>[2x]MVPISPIETVPVKLKPGMDGPKVKQWPLTEEKIKALVEICTEMEKEGKISKIGPENPYNTPVFACKKKDSTKWRKLVDFRELNKRTQDFWEVQLGIPHPAGLKKKKSVTVLDVGDAYFSVPLDEDFRKYTAFTIPSINNETPGIRYQYNVLPQGWKGSPAIFQSSMTKILEPFKKQNPDIVIYQYMDDLYVGSDLEIGQHRTKIEELRQHLLRWGLTTPDKKHQKEPPFLWMGYELHPDKWTVQPIVLPEKDSWTVNDIQKLVGKLNWASQIYPGIKVRQLSKLLRGTKALTEVIPLTEEAELELAENREILKEPVHGVYYDPSKDLIAEIQKQGQGQWTYQIYQEPFKNLKTGKYARMRGAHTNDVKQLTEAVQKITTESIVIWGKTPKFKLPIQKETWETWWTEYWQATWIPEWEFVNTPPLVKLWYQLEKEPIVGAETFYVDGAANRETKLGKAGYVTNKGRQKVVPLTNTTNQKTELQAIYLALQDSGLEVNIVTDSQYALGIIQAQPDKSESELVNQIIEQLIKKEKVYLAWVPAHKGIGGNEQVDKLVSA;>[2x]MAHHHHHHALEVLFQGPISPIETVPVKLKPGMDGPKVKQWPLTEEKIKALVEICTEMEKEGKISKIGPENPYNTPVFAIKKKDSTKWRKLVDFRELNKRTQDFWEVQLGIPHPAGLKKKKSVTVLDVGDAYFSVPLDEDFRKYTAFTIPSINNETPGIRYQYNVLPQGWKGSPAIFQSSMTKILEPFKKQNPDIVIYQYMDDLYVGSDLEIGQHRTKIEELRQHLLRWGLTTPDKKHQKEPPFLWMGYELHPDKWTVQPIVLPEKDSWTVNDIQKLVGKLNWASQIYPGIKVRQLSKLLRGTKALTEVIPLTEEAELELAENREILKEPVHGVYYDPSKDLIAEIQKQGQGQWTYQIYQEPFKNLKTGKYARMRGAHTNDVKQLTEAVQKITTESIVIWGKTPKFKLPIQKETWETWWTEYWQATWIPEWEFVNTPPLVKLWYQ

HIV-1 reverse transcriptase (RT) copies the viral ~10-kilobase ssRNA genome to a dsDNA in a multistep process. For the DNA synthesis, RT binds an eighteen-base-pair stretch of a duplex substrate with the primer 3′-end nucleotide occupying the priming site (P site). A dNTP complementing the first template overhang binds the N site and the nucleotide part is catalytically incorporated by RT at the 3′-end of the primer with the release of pyrophosphate. Following each nucleotide incorporation, the DNA is translocated from N to P site to accommodate the next dNTP.

Fragment 166, ((1 R,2 R)-2-phenyl-N-(1,3-thiazol-2-yl)) cyclopropanecarboxamide, occupies P-pocket. A comparison of the 166-bound structure with the RT/DNA P-1 complex structure with no compound bound, hereafter referred as the apo structure, shows the expansion of the pocket upon fragment binding. The deoxyribose ring of the primer 3′-end nucleotide has shifted by ~2.7 Å to accommodate 166. The five-membered thiazole moiety of 166 interacts with the deoxyribose ring and with the primer grip. The central cyclopropyl moiety is positioned over the conserved YMDD motif of the polymerase active site and interacting with the active-site residues Y183, M184, and D185. Consequently, the YMDD motif has bent down by ~1.6 Å compared with the apo structure. One Mg2+ ion that was chelating all three catalytic aspartates (D110, D185, and D186) in the apo structure, is dissociated upon binding of 166. The phenyl ring of 166 points toward the first template-overhang thymine base. This thymine base, which is less ordered in the apo structure due to lack of interaction, has shifted by ~2.2 Å and aligned with the phenyl ring of 166. Despite no canonical base-pairing or a typical hydrogen-bond interaction between the thymine base and the phenyl ring of 166, both aromatic rings are aligned and stacked against the dsDNA base pair, suggesting that modification of the phenyl ring of 166 to form base-pair-like interaction with the template base would improve binding. Compound 166 in P-pocket almost mimics the binding of a nucleotide and the predominant interaction of 166 is its stacking with the terminus base pair at the P-1 position.>[2x]MGSSHHHHHHSSGLVPRGSFQASMKHNI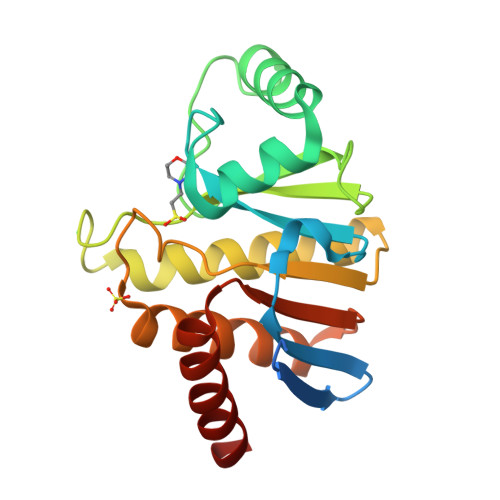NDNTLEIVVGDITKETTNVIVNAANGSLLGGGGVDGAIHHAAGPELLKACQEMRNNELNGEELPTGEVIITSGFQLPSRFIIHTVGPIWNQTPDLQEELLANCYRNALELVKVKKLSSISFPSISTGVYGYPIHEAAAIALQTIIQFLQENDVGLVKVVLFSERDYSIYQEKLKYLIEKI> LPEAYIPNAATEDERYYVPFTETVASRPLWISPQQNRWCDILLAREAGLVNRHYHPHEVFAYTISGKWGYLEHDWTATRGDFVYETPGEGHTLVAFEHEEP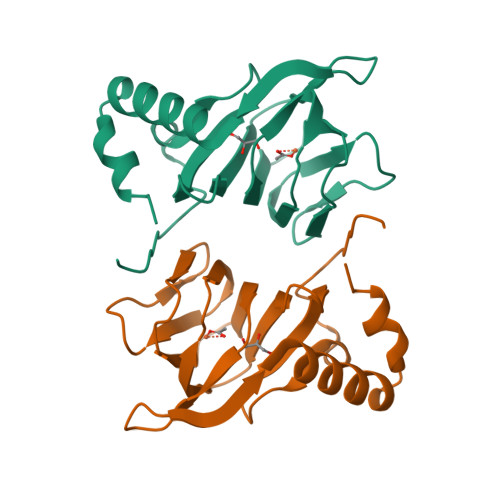MRVFFIVQGPLIWLDEAGNSIGHFDVHDYIAMCREHYEKVGLGADLVVTLFR>MKHHHHHHMHHHHHHENLYFQGWQENKSWNAHFTEHKSQGVVVLWNENKQQGFTNNLKRANQAFLPASTFKIPNSLIALDLGVVKDEHQVFKWDGQTRDIATWNRDHNLITAMKYSVVPVYQEFARQIGEARMSKMLHAFDYGNEDISGNVDSFWLDGGIRISATEQISFLRKLYHNKLHVSERSQRIVKQAMLTEANGDYIIRAKTGYSTRIEPKIGWWVGWVELDDNVWFFAMNMDMPTSDGLGLRQAITKEVLKQEK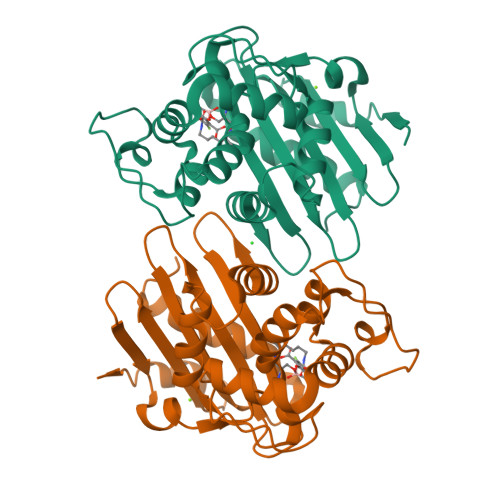IIP[4x]> MKYMITSKGDEKSDLLRLNMIAGFGEYDMEYDDVEPEIVISIGGDGTFLSAFHQYEERLDEIAFIGIHTGHLGFYADFRPAEADKLVKLLAKGEYQKVSYPLLKTTVKYGIGKKEATYLALNESTVKSSGGPFVVDVVINDIHFERFRGDGLCMSTPSGTTAYNKSLGGALMHPSIEAMQLTEMASINNRVYRTIGSPLVFPKHHVVSLQPVNDKDFQISVDHLSILHRDVQEIRYEVSAKKIHFARFRSFPFW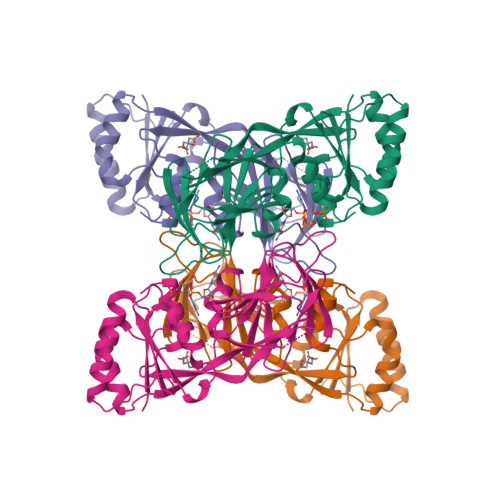RRVHDSFIEDLEHHHHHH>[2x]MDSDTDTDSGPVVATTKLVTFLQRVQHTALRSYPKKQTPDPKSYIDLSLKRPYSLSTIESAFDDLTSESHDQPVPVETLEKFVKEYFDGAGEDLLHHEPVDFVSDPSGFLSNVENEEVREWAREVHGLWRNLSCRVSDSVRESADRHTLLPLPEPVIIPGSRFREVYYWDSYWVIKGLMTSQMFTTAKGLVTNLMSLVETYGYALNGARAYYTNRSQPPLLSSMVYEIYNVTKDEELVRKAIPLLLKEYEFWNSGKHKVVIRDANGYDHVLSRYYAMWNKPRPESSVFDEESASGFSTMLEKQRFHRDIATAAESGCDFSTRWMRDPPNFTTMATTSVVPVDLNVFLLKMELDIAFMMKVSGDQNGSDRFVKASKAREKAFQTVFWNEKAGQWLDYWLSSSGEESETWKAENQNTNVFASNFAPIWINSINSDENLVKKVVTALKNSGLIAPAGILTSLTNSGQQWDSPNGWAPQQEMIVTGLGRSSVKEAKEMAEDIAR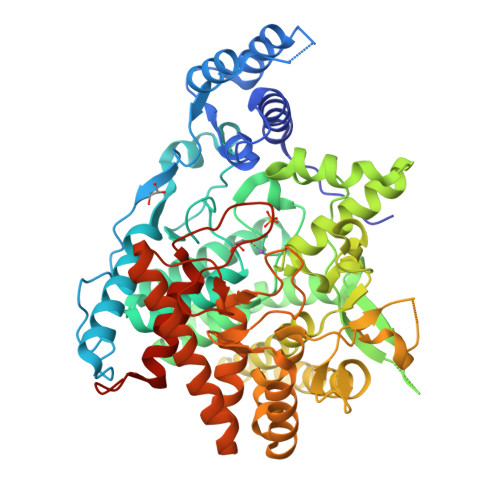RWIKSNYLVYKKSGTIHEKLKVTELGEYGGGGEYMPQTGFGWSNGVILAFLEEYGWPSHLSIEALEHHHHHH>MKDNTVPLKLIALLANGEFHSGEQLGETLGMSRAAINKHIQTLRDWGVDVFTVPGKGYSLPEPIQLLNAKQILGQLDGGSVAVLPVIDSTNQYLLDRIGELK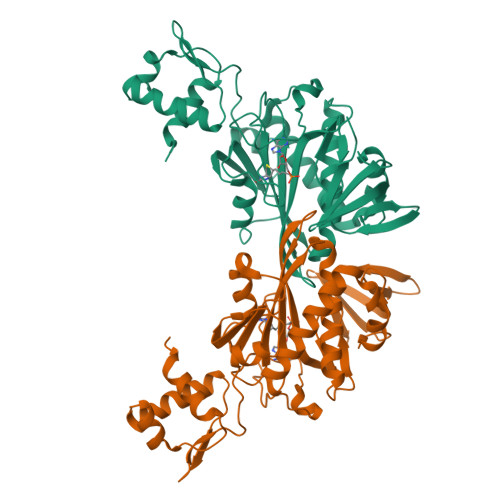SGDACIAEYQQAGRGRRGRKWFSPFGANLYLSMFWRLEQGPAAAIGLSLVIGIVMAEVLRKLGADKVRVKWPNDLYLQDRKLAGILVELTGKTGDAAQIVIGAGINMAMRRVEESVVNQGWITLQEAGINLDRNTLAAMLIRELRAALELFEQEGLAPYLSRWEKLDNFINRPVKLIIGDKEIFGISRGIDKQGALLLEQDGIIKPWMGGEISLRSAEK[2x]3-DEAZA-ADENOSINE 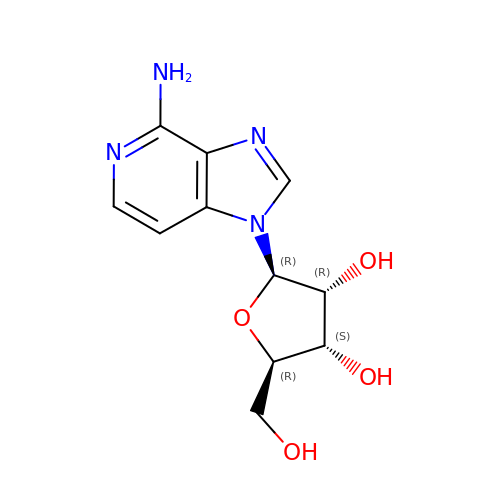| C11 H14 N4 O4 | DBZQFUNLCALWDY-PNHWDRBUSA-N Centrioles have proximal-distal polarity and a 9-fold radial symmetry imparted by a likewise symmetrical central scaffold, the cartwheel. The spindle assembly abnormal protein 6 (SAS-6) self-assembles into 9-fold radially symmetric ring-shaped oligomers that stack via an unknown mechanism to form the cartwheel. SAS-6 proteins comprise a globular “head” domain at their N-terminus followed by a long coiled coil that mediates stable protein homo-dimerization (Keller et al., 2014), and a disordered C-terminal extension. The characteristic shape of the SAS-6 ring led to the proposal that the protein head domains comprise the central “hub” of the centriolar cartwheel, with SAS-6 coiled coils forming the cartwheel “spokes” (Cottee et al., 2015; Kitagawa et al., 2011; van Breugel et al., 2011; van Breugel et al., 2014; Yoshiba et al., 2019).

Recombinantly produced fragments of the corresponding coiled-coil domains were folded, as judged by thermal denaturation experiments monitored by circular dichroism (CD) spectroscopy, and formed dimers in solution size exclusion chromatography–multiangle light scattering (SEC-MALS) assays. We succeeded in crystalizing a fragment of the coiled-coil domain from each species, with different boundaries, but spanning approximately the middle one-third of this protein region (henceforth, CrSAS-6_CCMiddle, DrSAS-6_CCMiddle, and HsSAS-6_CCMiddle; see Figure S2A for the protein sequence alignment, Table 1 for a list of recombinant protein constructs, and Figure S1A for SDS-PAGE analysis of these constructs). As the HsSAS-6_CCMiddle and DrSAS-6_CCMiddle fragments did not originally include methionine residues, one or two amino acids, respectively, were mutated to methionine to allow SeMet incorporation. All three SAS-6 structures revealed two-stranded parallel coiled-coil domains as analyzed by SOCKET, in agreement with the predicted nature of this protein section. Only parallel associations between coiled-coil domains are compatible with the stacking of SAS-6 rings into a continuous cartwheel, whereas antiparallel coiled-coil interactions would lead to horizontal displacement of SAS-6 rings, a distribution incompatible with a stacked rings configuration. Both the HsSAS-6_CCMiddle and DrSAS-6_CCMiddle crystal structures revealed primarily antiparallel associations between their coiled coils, with only much smaller parallel associations between coiled-coil copies, which were offset by approximately one-half length or the full length of the crystallographic c-axis, respectively. A previous hypothesis posited that STIL/SAS-5/Ana2, an essential centriolar component that forms higher-order oligomers (Cottee et al., 2015; David et al., 2016; Rogala et al., 2015; Shimanovskaya et al., 2013) and binds to SAS-6 (Dzhindzhev et al., 2014; Hilbert et al., 2013; Ohta et al., 2014; Qiao et al., 2012), could cross-link SAS-6 copies, thereby stabilizing SAS-6 oligomer formation and their 3D arrangement.

>GPLESSHHRSTQQLQTKVSELETANRELIDKKYKSDSTIRDLKAKMTSLEEECQRSKQQVLSLRRENSALDSECHEKERLMNQLQTRVAVLEQEIKDKDQLVLRTKEVLEATQQQKNS[4x]>[2x]SMDPERRVRSTLKKVFGFDSFKTPLQESATMAVVKGNKDVFVCMPTGAGKSLCYQLPALLAKGITIVVSPL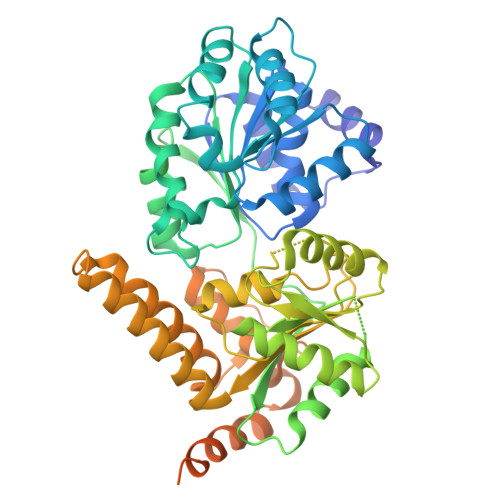IALIQDQVDHLLTLKVRVSSLNSKLSAQERKELLADLEREKPQTKILYITPEMAASSSFQPTLNSLVSRHLLSYLVVDEAHCVSQWGHDFRPDYLRLGALRSRLGHAPCVALTATATPQVQEDVFAALHLKKPVAIFKTPCFRANLFYDVQFKELISDPYGNLKDFCLKALGQEADKGLSGCGIVYCRTREACEQLAIELSCRGVNAKAYHAGLKASERTLVQNDWMEEKVPVIVATISFGMGVDKANVRFVAHWNIAKSMAGYYQESGRAGRDGKPSWCRLYYSRNDRDQVSFLIRKEVAKLQEKRGNKASDKATIMAFDALVTFCEELGCRHAAIAKYFGDALPACAKGCDHCQNPTAVRRRLEALERSSSWSKTCIGPSQGNGFDPELYEGGRKGYGDFSRYDEGSGGSGDEGRDEAHKREWNLFYQKQMQLRKGKDPKIEEFV> GRAEGLGGLERFCSPGKGRGLRALQPFQVGDLLFSCPAYAYVLTVNERGNHCEYCFTRKEGLSKCGRCKQAFYCNVECQKEDWPMHKLECSPMVVFGENWNPSETVRLTARILAKQKIHPERTPSEKLLAVKEFESHLDKLDNEKKDLIQSDIAALHHFYSKHLGFPDNDSLVVLFAQVNCNGFTIEDEELSHLGSAIFPDVALMNHSCCPNVIVTYKGTLAEVRAVQEIKPGEEVFTSYIDLLYPTEDRNDRLRDSYFFTCECQECTTKDKDKAKVEIRKLSDPPKAEAIRDMVRYARNVIEEFRRAKHYKSPSELLEICELSQEKMSSVFE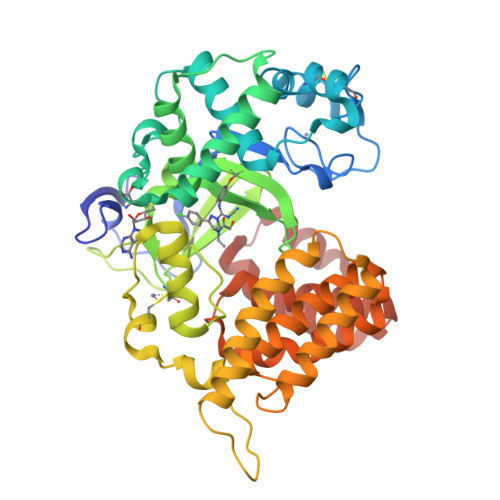DSNVYMLHMMYQAMGVCLYMQDWEGALQYGQKIIKPYSKHYPLYSLNVASMWLKLGRLYMGLEHKAAGEKALKKAIAIMEVAHGKDHPYISEIKQEIESH> KLSEHLRYCDSILREMLSKK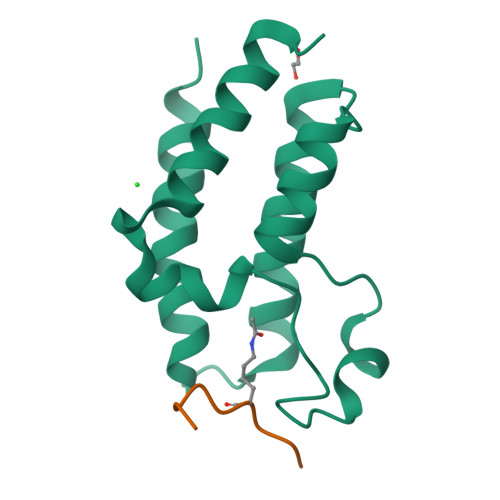HAAYAWPFYKPVDAEALELHDYHDIIKHPMDLSTVKRKMDGREYPDAQGFAADVRLMFSNCYKYNPPDHEVVAMARKLQDVFEMRFAKMP;> APRKQLATK>[3x]GIEIVNRKAVWYLTSEIKETETGIEVSAGELHKGDEEVFPVEEVSFDLTPDDTYPVEY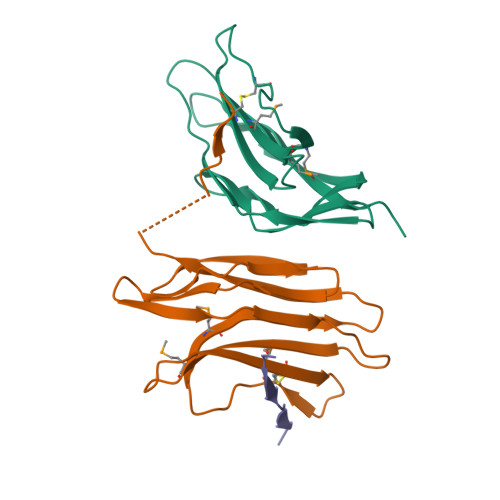MLYLHMNVQTKKVSWSLCKAYLDGEGYCDYQGNERLIMYPVSVTVFPNGTREGTIFLYEKEDREPDRKPPVIVEPQPVGEIGTPDIDE>MASMREDYSLECDPAVIGTAVKGKEAVHSDLGYWIESEKNDTWRLKRAHLIEMKTCEWPKSHTLWTDGIEESDLIIPKSLAGPLSHHNTREGYRTQMKGPWHSEE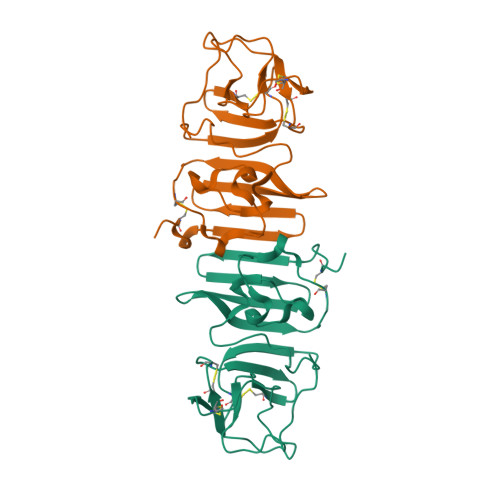LEIRFEECPGTKVHVEETCGTRGPSLRSTTASGRVIEEWCCRECTMPPLSFRAKDGCWYGMEIRPRKEPESNLVRSMVTA[2x]>[2x]MIPGKPFDTPQLAAELERWKLDGRDVSLLIGGPEGLSPACKAAAEQSWSLSALTLPHPLVRVLVAESLYRAWSITTNHPYHREGSMKLQLVAVGTKMPDWVQTGFTEYLRRF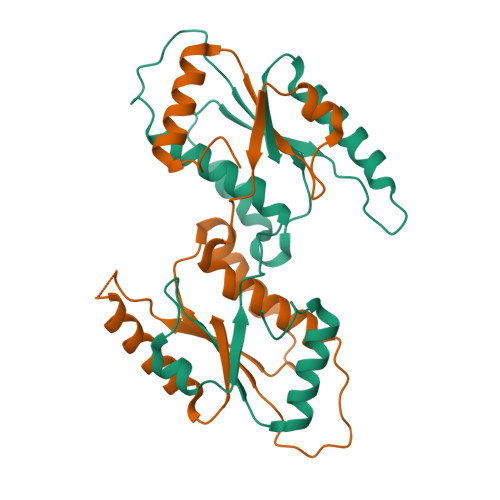PKDMPFELIEIPAGKRGKNADIKRILDKEGEQMLAAAGKNRIVTLD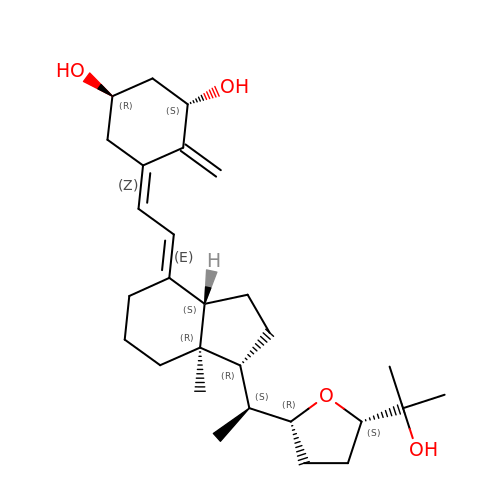(1~{R},3~{S},5~{Z})-5-[(2~{E})-2-[(1~{R},3~{a}~{S},7~{a}~{R})-7~{a}-methyl-1-[(1~{S})-1-[(2~{R},5~{S})-5-(2-oxidanylpropan-2-yl)oxolan-2-yl]ethyl]-2,3,3~{a},5,6,7-hexahydro-1~{H}-inden-4-ylidene]ethylidene]-4-methylidene-cyclohexane-1,3-diol | C28 H44 O4 | DDIWZQGTNVZJGO-GKBMNYJXSA-N~{N}-[(4-fluorophenyl)methyl]-4-methoxy-aniline | C14 H14 F N O | 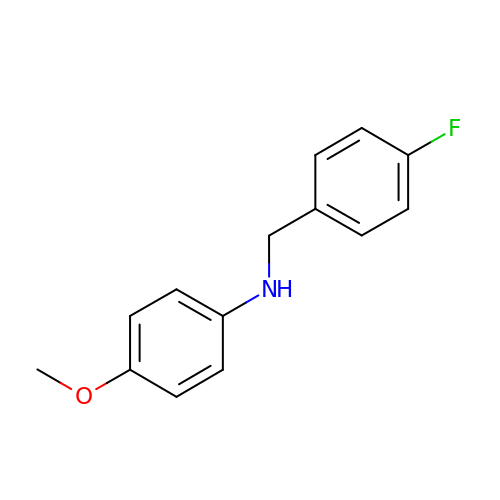QHNUQKUZGHGTCA-UHFFFAOYSA-N> SNACTRAVYLGPDRMVVTGRTMDWKEDIMSNIYVFPRGMQRAGHNKEKTVNWTSKYGSVIATGYDIGTCDGMNEKGLVASLLFLPESVYSLPGDTRPAMGISIWTQYVLDNFATVREAVDEMKKETFRIDAPRMPNGGPESTLHMAITDETGNTAVIEYLDGKLSIHEGKEYQVMTNSPRYELQLAVNDYWKEVGGLQMLPGTNRSSDRFVRASFYIHAIPQTADAKIAVPSVLSVMRNVSVPFGINTPEKPHISSTRWRSVSDQKNKVYYFESTLTPNLFWLDLKKIDF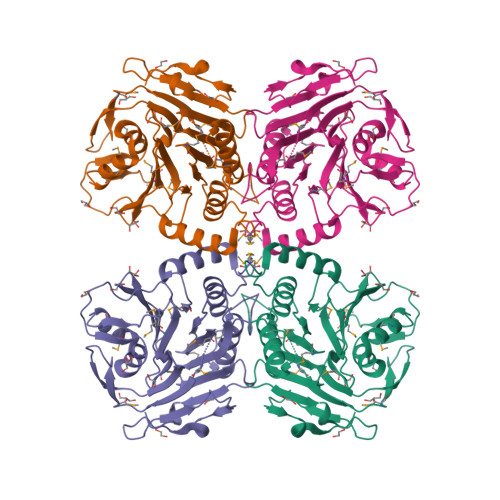SPKAGVKKLSLTKGEIYAGDAVKDLKDSQS> MSERIVISPTSRQEGHAELVMEVDDEGIVTKGRYFSITPVRGLEKMVTGKAPETAPVMVQRICGVCPIPHTLASVEAIDDSLDIEVPKAGRLLRELTLAAHHVNSHAIHHFLIAPDFVPENLMADAINSVSEIRKNAQYVVDMVAGEGIHPSDVRIGGMADNITELARKRLYARLKQLKPKVNEHVELMIGLIEDKGLPEGLGVHNQPTLASHQIYGDRTKFDLDRFTEIMPESWYDDPEIAKRACSTIPLYDGRNVEVGPRARMVEFQGFKERGVVAQHVARALEMKTALSRAIEILDELDTSAPVRADFDERGTGKLGIGAI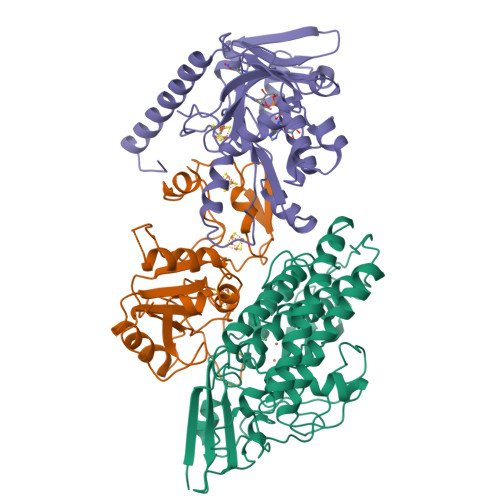EAPRGLDVHMAKVENGKIQFYSALVPTTWNIPTMGPATEGFHHEYGPHVIRAYDPCLSCATHVMVVDDEDKSVIKNEMVKI;> MSLIARIKRFLGLEAEAKREEPEKEKSEPVGASKEEVEKVAEENAKPRIGYIHLSGCTGDAMSLTENYDILAELLTNMVDIVYGQTLVDLWEMPEMDLALVEGSVCLQDEHSLHELKELREKAKLVCAFGSCAATGCFTRYSRGGQQAQPSHESFVPIADLIDVDLALPGCPPSPEIIAKTVVALLNNDMDYLQPMLDLAGYTEACGCDLQTKVVNQGLCIGCGTCAMACQTRALDMTNGRPELNSDRCIKCGICYVQCPRSWWPEEQIKKELGL;> MVLGTYKEIVSARSTDREIQKLAQDGGIVTGLLAYALDEGIIEGAVVAGPGEEFWKPQPMVAMSSDELKAAAGTKYTFSPNVMMLKKAVRQYGIEKLGTVAIPCQTMGIRKMQTYPFGVRFLADKIKLLVGIYCMENFPYTSLQTFICEKLGVSMELVEKMDIGKGKFWVYTQDDVLTLPLKETHGYEQAGCKICKDYVAELADVSTGSVGSPDGWSTVITRTDAGDSIFKQAVEAGLFETKPIEEVKPGLGLLEKLAAQKKEKAEKNIAARKEMGLPTPF The Ca2+/calmodulin(CaM)-dependent protein kinase II (CaMKII) α isoform is a central mediator of synaptic plasticity that underlies learning, memory and cognition. A hallmark feature of CaMKII regulation is autophosphorylation at T286, which generates Ca2+/CaM-independent ‘autonomous’ kinase activity that persists even when the initial Ca2+-stimulus subsides. The principle domain sequence of a CaMKII subunit is illustrated in, with an N-terminal kinase domain, followed by a short regulatory domain that contains T286, the variable linker domain that is subject to alternative splicing, and the C-terminal hub domain.

A 3D EM density map was obtained at 20 Å resolution by using a combination of tilted-series tomographic imaging and 3D masking routines. The central density of the EM map is well defined by the crystal structure of the dodecameric hub complex, formed by residues 345–472 (cross-correlation=0.95 at 20 Å resolution). The structured N-terminal kinase/regulatory domain, containing residues 13–300, was best fit computationally into each of the radial densities with the regulatory domain (red ribbon in Fig. 2a) oriented towards the central hub complex (cross-correlation=0.98 at 20 Å resolution). Therefore, for the basal-state holoenzyme structure determined here, each N-terminal kinase/regulatory domain was covalently connected to the nearest C-terminal hub domain by a random coil peptide chain, containing residues 301–344 (red and grey coil). The pseudo-atomic model presented here provides a representative average view of the CaMKIIα holoenzyme in an extended (and activatable) conformation. In this form of the holoenzyme, the kinase domains are arranged independently from each other and removed from the central hub complex. Each kinase domain is separated from the central hub complex, extending the radius of the model to ∼135 Å. Neighbouring kinase domains are separated from each other by ∼60 Å (center-to-center distance). In this extended form of the holoenzyme, the CaM-binding sites (residues 294–314, red ribbon/coil) are solvent exposed and thus positioned for activation by the Ca2+/CaM-stimulus. Single particle analysis revealed a high degree of flexibility for kinase domain positioning, with almost none of the individual particles completely matching the average structure.

>[12x]MYQLFEELGKGAFSVVRRCVKVLAGQEYAAKIINTKKLSARDHQKLEREARICRLLKHPNIVRLHDSISEEGHHYLIFDLVTGGELFEDIVAREYYSEADASHCIQQILEAVLHCHQMGVVHRDLKPENLLLASKLKGAAVKLADFGLAIEVEGEQQAWFGFAGTPGYLSPEVLRKDPYGKPVDLWACGVILYILLVGYPPFWDEDQHRLYQQIKAGAYDFPSPEWDTVTPEAKDLINKMLTINPSKRITAAEALKHPWISHRSTVASCMHRQETVDCLKKFNARRKLKGAILTTMLATRNFSGGKSGGNKKSDGVKESSESTNTTIEDEDTKVRKQEIIKVTEQLIEAISNGDFESYTKMCDPGMTAFEPEALGNLVEGLDFHRFYFENLWSRNSKPVHTTILNPHIHLMGDESACIAYIRITQYLDAGGIPRTAQSEETRVWHRRDGKWQIVHFHRSGA> MLITDTLSPQAFEEALRAKGDFYHIHHPYHIAMHNGNATREQIQGWVANRFYYQTTIPLKDAAIMANCPDAQTRRKWVQRILDHDGSHGEDGGIEAWLRLGEAVGLSRDDLLSERHVLPGVRFAVDAYLNFARRACWQEAACSSLTELFAPQIHQSRLDSWPQHY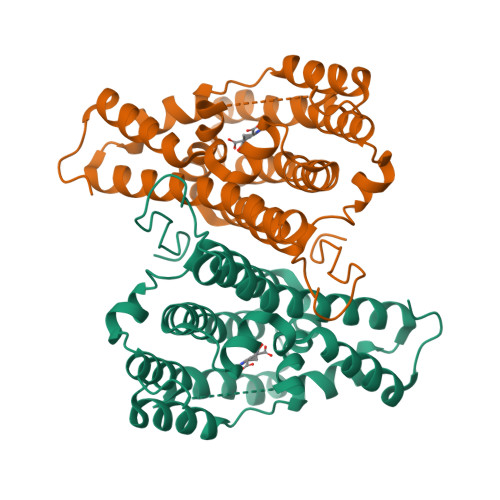PWIKEEGYFSFRSSLSQANRDVEHGLALAKAYCDSAEKQNRMLEILQFKLDILWSMLDAMTMAYALQRPPYHTVTDKAAWHTTRLVLEHHHHH>[2x]AAPTAIEHMEPPFWWAGMQHKGLQLMVHGRDIGRMEAALDYPGVRLVSPTRVPNANYLFVDLEIGPEAQPGSFDIVFKGDGRSERYRYRLLAREQGSAQRQGFGPGDAIYQIMPDRFANGDPSNDNVAGMREQADRRHGGGRHGGDIRGTIDHLDYIAGLGFTQLWPTPLVENDAAAYSYHGYAATDHYRIDPRYGSNEDFVRLSTEARKRGMGLIQDVVLSHIGKHHWWMKDLPTPD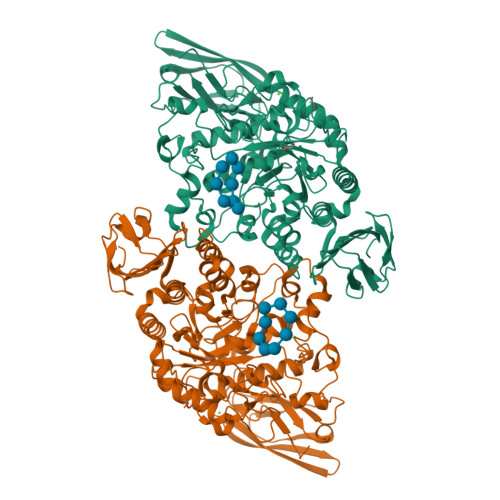WINYGGKFVPTQHHRVAVQDPYAAQADSENFTKGWFVEGMPDLNQTNPLVANYLIQNNIWWIEYAGLSGLRIDTYGYSDGAFLTEYTRRLMAEYPRLNMVGQEWSTRVPVVARWQRGKANFDGYTSHLPSLMDFPLVDAMRNALSKTGEENGLNEVYETLSLDYLYPEPQNLVLFGGNHDMARMFSAAGEDFDRWRMNLVFLMTMPRIPQFYSGDEILMTSTVKGRDDASYRRDFPGGWAGDKANAFSGAGLTSQQRAAQDLVRKLANWRKNQPVIHNGRLMHFGPEENTWVYFRYNKDKRIMVAMNNNDKPMTLPTARFQEMLKGAPSGVDFLSGKTVGLGRELRLAPKSVVVIELPGLPEA>[2x]MNKPQLPDFIQNKIDHYIENYFDINKNGKHLVLGKQASPDDIILQSNDYLALANHPLIKARLAKSLLEEQQSLFMSASFLQNDYDKPMIEKRLAKFTGFDECLLSQSGWNANVGLLQTICQPNTN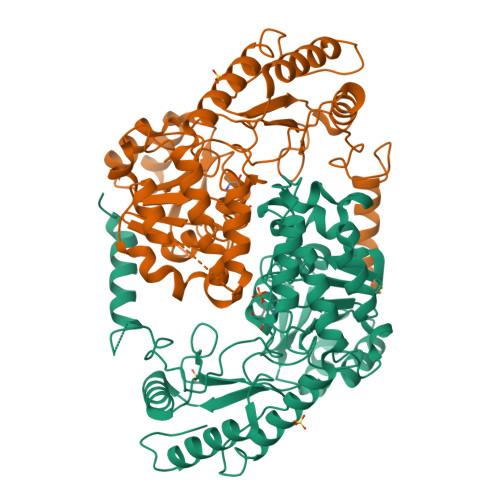VYIDFFAHMSLWEGARYANAQAHPFMHNNCDHLRMLIQRHGPGIIVVDSIYSTLGTIAPLAELVNISKEFGCALLVDESHSLGTHGPNGAGLLAELGLTREVHFMTASLAKTFAYRAGAIWCNNEVNRCVPFISYPAIFSSTLLPYEAAGLETTLEIIESADNRRQHLDRMARKLRIGLSQLGLTIRSESQIIGLETGDERNTEKVRDYLESNGVFGSVFCRPATSKNKNIIRLSLNSDVNDEQIAKIIEVCSDAVNYGDFYFR>MSQSIEEKSVQERTRIKNSRYESGVIPYAKMGYWNPDYQVKDTDVLALFRVTPQPGVDPIEAAAAVAGESSTATWTVVWTDLLTAADLYRAKAYKVDQVPNNPEQYFAYIAYELDLFEEGSIANLTASIIGNVFGFKAVKALRLEDMRLPLAYLKTFQGPATGVILERERLDKFGRPLLGCTTKPKLGLSGKNYGRVVYEALKGGLDFVKDDENINSQPFMRWRERYLFTMEAVNKASAATGEVKGHYLNVTAATMEEMYARANFAKELGSVIIMIDLVIGYTAIQTMAKWARDNDMILHLHRAGNSTYSRQKNHGMNFRVICKWMRMAGVDHIHAGTVVGKLEGDPIITRGFYKTLLLPKLERNLQEGLFFDMEWASLRKVMPVASGGIHAGQMHQLIHYLGEDVVLQFGGGTIGHPDGIQAGATANRVALEAMILARNENRDYLTEGPEILREAAKTCGALRTALDLWKDITFNYTSTDTSDFVETPTANI[4x];>VRITQGTFSFLPDLTDEQIKKQIDYMISKKLAIGIEY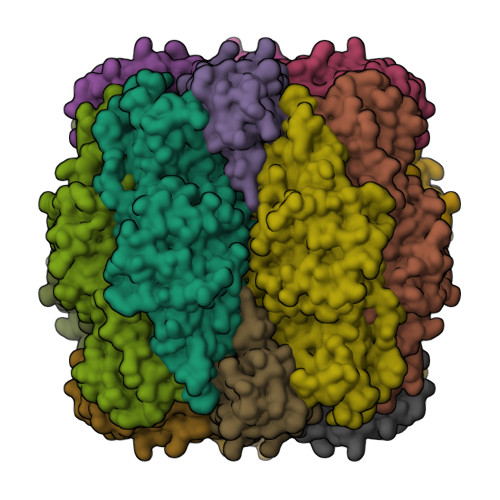TNDIHPRNAYWEIWGLPLFDVTDPAAVLFEINACRKARSNFYIKVVGFSSVRGIESTIISFIVNRPKHEPGFNLMRQEDKSRSIKYTIHSYESYKPEDERY[4x]{4-[2-ACETYLAMINO-2-(3-CARBAMOYL-2-CYCLOHEXYLMETHOXY-6,7,8,9-TETRAHYDRO-5H-BENZOCYCLOHEPTEN-5YLCARBAMOYL)-ETHYL]-2-PHOSPHONO-PHENYL}-PHOSPHONIC ACID | C30 H41 N3 O10 P2 | 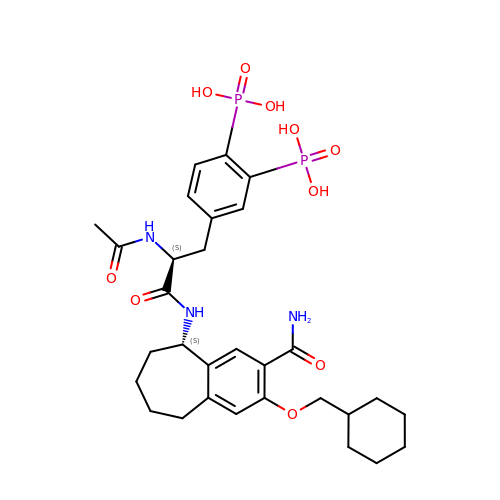SPSGYTWOIGAABK-DQEYMECFSA-N>[2x]MRIVEVYSHLNGLEYIQVHLPHIWEEIQEIIVSIDAEACRTKESKEKTKQGQILYSPVALNEAFKEKLEAKGWKESRTNYYVTADPKLIRETLSLEPEEQKKVIEA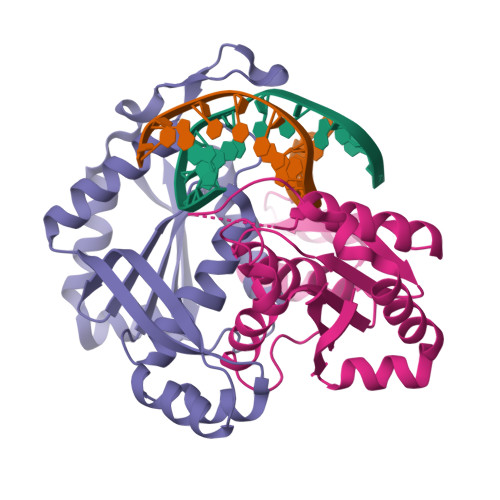AGKEALKSYNQTDFVKDRVAIEVQFGKYSFVAYDLFVKHMAFYVSDKIDVGVEILPMKELSKEMSSGISYYEGELYNVIRQGRGVPAVPLVLIGIAP(9Z)-11-{(2R,3S)-3-[(2Z)-pent-2-en-1-yl]oxiran-2-yl}undec-9-enoic 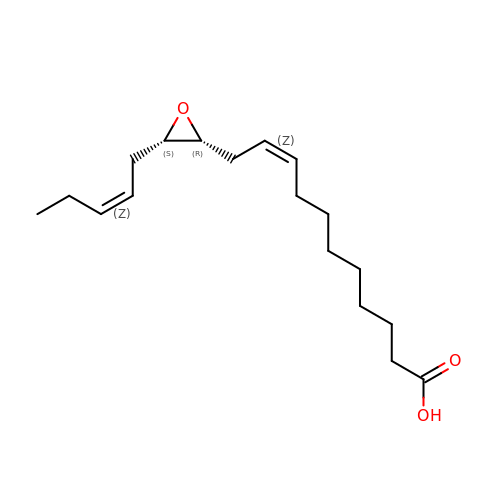acid | C18 H30 O3 | BKKGUKSHPCTUGE-ZQCGFPFMSA-N4-[2-fluoro-6-(trifluoromethyl)anilino]-2-[(6-methoxy-2-methyl-1,2,3,4-tetrahydroisoquinolin-7-yl)amino]pyrimidine-5-carboxamide 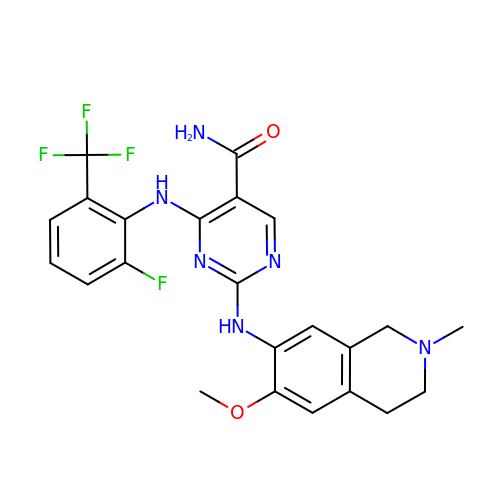| C23 H22 F4 N6 O2 | RZLXOEIALAVGKH-UHFFFAOYSA-N> SGVDDDMACHKIPVEADFLYAYSTAPGYYSWRNSKDGSWFIQSLCAML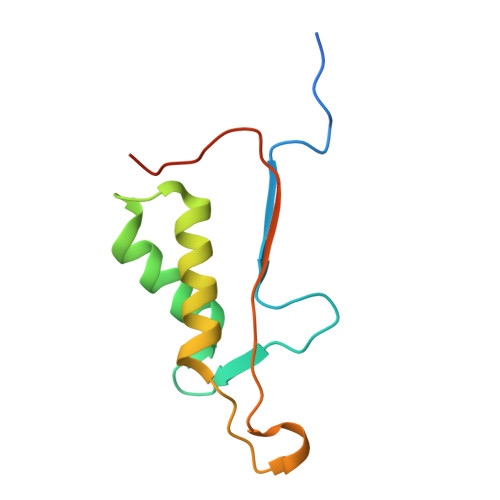KQYADKLEFMHILTRVNRKVATEFESFSFDATFHAKKQIPCIVSMLTKELYFYHHHHHH>[2x]MNHKVHHHHHHIEGRHMRILFFSSQAYDSESFQASNHRHGFELHFQQAHLQADTAVLAQGFEVVCAFVNDDLSRPVLERLAAGGTRLVALRSAGYNHVDLAAAEALGLPVVHVPAYSPHAVAEHAVGLILT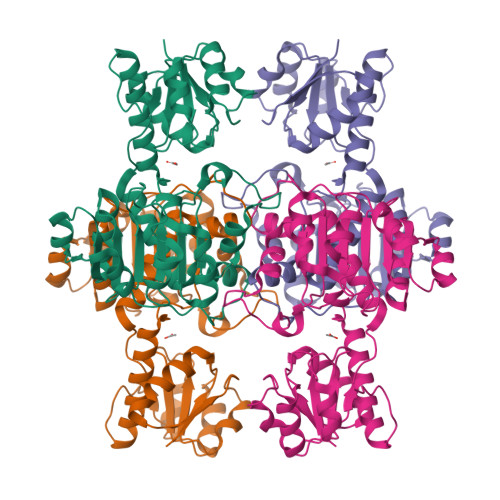LNRRLHRAYNRTREGDFSLHGLTGFDLHGKRVGVIGTGQIGETFARIMAGFGCELLAYDPYPNPRIQALGGRYLALDALLAESDIVSLHCPLTADTRHLIDAQRLATMKPGAMLINTGRGALVNAAALIEALKSGQLGYLGLDVYEEEADIFFEDRSDQPLQDDVLARLLSFPNVVVTAHQAFLTREALAAIADTTLDNIAAWQDGTPRNRVRA Replication Protein A (RPA) is a heterotrimeric single stranded DNA-binding protein with essential roles in DNA replication, recombination and repair. In Archaea, the same function is also fulfilled by a heterotrimeric RPA. We report three crystal structures and five cryo-EM structures of Pyrococcus abyssi RPA (hereafter referred to PabRPA), in its apo form as well as bound to ssDNA. We find that archaeal and eukaryotic RPAs share a conserved heterotrimerization core, which is composed of three OB domains connected through a three-helix bundle formed by a C-terminal α-helix from each subunit.

We biochemically reconstituted, crystallized and determined the 3.7 Å X-ray crystal structure of a heterotrimeric complex of P. abyssi Rpa1, Rpa2, and Rpa3 subunits. Most of Rpa1 (2–358), Rpa2 (1–184), and Rpa3(6-117) subunits have been modeled in the electron density map, the only flexible region being the C-terminus of Rpa2 (185–268). PabRPA contains four OB domains, named OB-1, OB-2, OB-3, and OB-4, which share the highest structural similarity with OB-A, OB-C, OB-D and OB-E in eukaryotic RPA, respectively. Like in its eukaryotic OB-C counterparts, PabRPA OB-2 contains a Zn-finger motif that is inserted between β-strands β1 and β2, and a short helical domain that is inserted between β-strands β3 and β4. The Tri-C adopts a compact quaternary structure consisting of OB-2 of Rpa1, OB-3 of Rpa2, and OB-4 of Rpa3, which is the smallest subunit. Similar to the eukaryotic RPA, heterotrimerization of PabRPA is primarily mediated through a three-helix bundle formed by a C-terminal α-helix from each subunit. The trimerization helix of Rpa2 is followed by a helix-turn-helix motif, which stabilizes the Tri-C by extending the contacts between the Rpa2 and Rpa3 subunits. The N-terminal region of Rpa1 hosts two independent domains, which adopt an extended conformation in contrast to the compact structure of the Tri-C: the OB-1 DNA-binding domain and an archaea-specific helical domain named AROD (Acidic Rpa1 OB-binding Domain). Interestingly, in the PabRPA crystal structure, the tri-helical bundle simultaneously stacks against the OB-4 and OB-1 domains of the neighboring Rpa3 and Rpa1 chains, respectively, through a crystal lattice contact. Interestingly, the same OB-3/OB-3 interaction forms a crystal-packing contact in the crystal structure of full-length PabRPA in its apo form.

> MSVLTKDRIIEIIERKTGMSREEIEEEIRKIMEEDPYLSEQGAAALLAERLGIDLIEKEEVSLMRISELYPGMDPREVNVVGRVLKKYPPREYTRKDGSVGRVASLIIYDDSGRARVVLWDAKVSEYYNKIEVGDVIKVLDAQVKESLSGLPELHINFRARIILNPDDPRVEMIPPLEEVRVATYTRKKIKDIEAGDRFVEVRGTIAKVYRVLTYDACPECKKKVDYDEGLGVWICPEHGEVQPIKMTILDFGLDDGTGYIRVTLFGDDAEELLGVSPEEIAEKIKELEESGLTTKEAARKLAEDEFYNIIGREIVVRGNVIEDRFLGLILRASSWEDVDYRREIERIKEELEKLGVM;> MSKKRMPATRLYIKDILEGYFVKSEGDFEPNYLITKYARKVYRAKIVGTVVREPLIAEDETYGKFQVDDGTGVIWVLGFRDDTKFAKLVRKGDLVQVIGKIAEWRDDKQILVEGVSKVHPNMWILHRYETLKEKIEHIKKAKIALEIYNQYGITAKSKVIAKNKGIEEELLEVIDELYGIMMEERSIEEPMEELLEEEIPEEKEENELLEKAKEDILNILRQKRTAISRKYILKKLGDKYDEETIDDAITELLAQGEIYEPETGYYKL;> GTGDGSEVQVRRRKPAVERKISEIREEDTRVSLIGRVIKVDKMDYMFWLDDGTGVAIIESESDLPKVGQVVRVIGRIIRNEEGIHIYAEVIQDFSDADLEALEEIRELERKLLPRLEGEIVW> MNSPISPIETVPVKLKPGMDGPKVKQWPLTEEKIKALVEICTEMEKEGKISKIGPENPYNTPVFAIKKKDSTKWRKLVDFRELNKRTQDFWEVQLGIPHPAGLKKKKSVTVLDVGDAYFSVPLDEDFRKYTAFTIPSINNETPGIRYQYNVLPQGWKGSPAIFQSSMTKILEPFRKQNPDIVIYQYMDDLYVGSDLEIGQHRTKIEELRQHLLRWGLTTPDKKHQKEPPFLWMGYELHPDKWTVQPIVLPEKDSWTVNDIQKLVGKLNWASQIYPGIKVRQLCKLLRGTKALTEVIPLTEEAELELAENREILKEPVHGVYYDPSKDLIAEIQKQGQGQWTYQIYQEPFKNLKTGKYARMRGAHTNDVKQLTEAVQKITTESIVIWGKTPKFKLPIQKETWETWWTEYWQATWIPEWEFVNTPPLVKLWYQLEKEPIVGAETFYVDGAANRETKLGKAGYVTNRGRQKVVTLTDTTNQKTELQAIYLALQDSGLEVNIVTDSQYALGIIQAQPDQSESELVNQIIEQLIKKEKVYLAWVPAHKGIGGNEQVDKLVSAGIRKVL;> MNSPISPIETVPVKLKPGMDGPKVKQWPLTEEKIKALVEICTEMEKEGKISKIGPENPYNTPVFAIKKKDSTKWRKLVDFRELNKRTQDFWEVQLGIPHPAGLKKKKSVTVLDVGDAYFSVPLDEDFRKYTAFTIPSINNETPGIRYQYNVLPQGWKGSPAIFQSSMTKILEPFRKQNPDIVIYQYMDDLYVGSDLEIGQHRTKIEELRQHLLRWGLTTPDKKHQKEPPFLWMGYELHPDKWTVQPIVLPEKDSWTVNDIQKLVGKLNWASQIYPGIKVRQLCKLLRGTKALTEVIPLTEEAELELAENREILKEPVHGVYYDPSKDL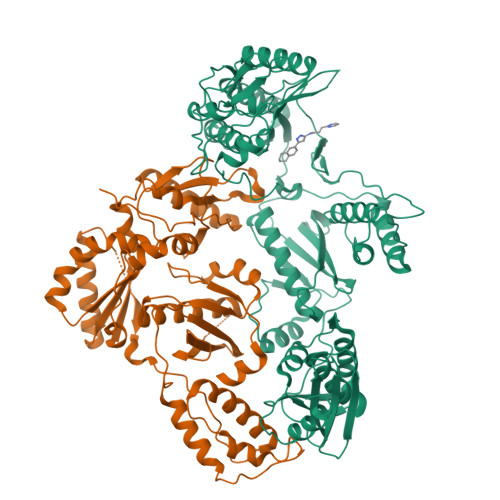IAEIQKQGQGQWTYQIYQEPFKNLKTGKYARMRGAHTNDVKQLTEAVQKITTESIVIWGKTPKFKLPIQKETWETWWTEYWQATWIPEWEFVNTPPLVKLWYQLEKEPIVGAETF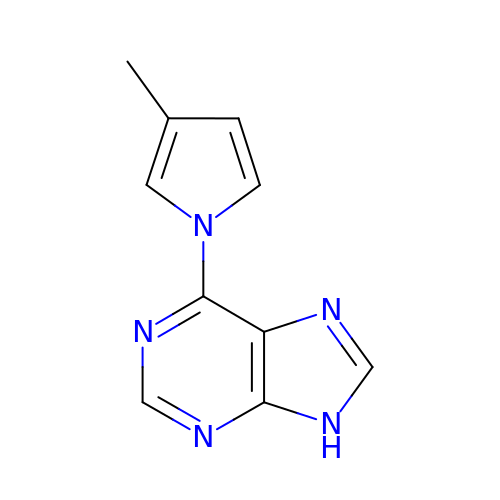6-(3-methyl-1H-pyrrol-1-yl)-9H-purine | C10 H9 N5 | BCVQNVIMHTYJMD-UHFFFAOYSA-N> VEEIKNASIK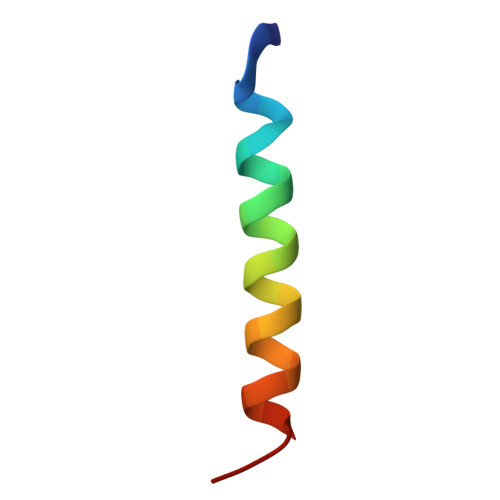RKLFGLANTIREQALE>MKKLLPILIGLSLTGFSAMSQAENLLQVYQQARISNPDLRKSAADRDAAFEKINEARSPLLPQLGLGADYTYTSGFRDYKDQNSNVTSGSLQLTQVLFDMSKWRALTLQEKAAGIQDVTYQTDQQTLILNTATAYFKVLAAIDTLSYTEAQKQAIYRQLDQTTQRFNVGLVAITDVQNARSQYDAVLANEVTARNDLDNAVEELRQVTGNYYPELASLNVDGFKTSKPQAVNALLKEAENRNLSLLQARLNQDLAREQIRQAQDGHLPTLDLNASSGVSNNRYSGSKSISQDADIGQNKIGLSFSLPLYQGGMVNSQVKQAQYNFVGASEQLESAHRSVVQTVRSSFNNVNASISSINAYKQAVVSAQSSLDAMEAGYSVGTRTIVDVLDATTTLYNAKQQLSNARYNYLINELNIKSALGTLNEQDLIALNNTLGKPISTSADSVAPENPQQDATADGYGNTTAAMKPASARTTTHSSGSNPFRQLEHHHHHH[3x];> MADNQPVPLTPAPPGMVSLGVNENGEEEMTVIGGDGSGTGFSGNEAPIIPGSGSLQADLGKKSLTRLQAESSAAIHATAKWTTENLAKTQAAQAERAKAAMLSQQAAKAKQAKLTQHLKDVVDRALQNNKTRPTVIDLAHQNNQQMAAMAEFIGRQKAIEEARKKAEREAKRAEEAYQAALRAQEEEQRKQAEIERKLQEARKQEAAAKAKAEADRIAAEKAEAEARAKAEAERRKAEEARKALFAKAGIKDTPGCLEHHHHHH

Here, we use biochemical, biophysical and structural analyses to show how a bacteriocin exploits TolC, a major outer-membrane antibiotic efflux channel in Gram-negative bacteria, to transport itself across the outer membrane of target cells. Klebicin C (KlebC), a rRNase toxin produced by Klebsiella pneumoniae, binds TolC of a related species (K. quasipneumoniae) with high affinity through an N-terminal, elongated helical hairpin domain common amongst bacteriocins. TolC is one of the most prevalent drug efflux channels in bacteria and is frequently associated with multidrug resistance. Our results indicate that TolC, in addition to its known role in antibiotic export, can function as a protein import channel for bacteriocins.

Application of symmetry during processing then allowed for symmetry expansion of the dataset and subtraction of particles to give a single monomer, after which 3D sorting of particles revealed several classes where KlebC density was weakly apparent. A single class was further processed (see “Methods” and Supplementary Fig. 5) to produce the final 3.1 Å map of the TolC trimer with both helix 1 and 2 of KlebC resolved. In the final model, density corresponding to helix 1 and the N-terminal end of helix 2 of a single KlebC molecule span 109 Å of the TolC lumen; the N-terminal end of helix 1 is located near the periplasmic iris of TolC while helix 2 resides near the top within the outer-membrane β-barrel. The conformation of KlebC observed within the complex demonstrates unequivocally that the KlebC hairpin unfurls, forming a distorted kinked structure in which helix 1 is positioned against the α-helical region of TolC, and residues 137–151 form helix 2 within the transmembrane β-barrel of TolC. By contrast, in the complex with KqTolC this region forms the N-terminal end of helix 2. In contrast, helix 2 of KlebC packs against the β-barrel region of chain C with His140 and Gln141, from within interhelical linker, now forming hydrogen bonds to Ser68 and Asp47 of TolC, respectively. The N-terminus of KlebC helix 1 is oriented such that it is proximal to both chain A and C of the TolC trimer towards the iris, whilst the C-terminus of helix 1 can solely interact with chain A where the helices of TolC meet the β-barrel strands at the inner leaflet of the OM. The modelled structure of the complex shows charge complementarity plays an important role in stabilising the complex since several localised regions of positive and negative charge are matched. The unfurling of the KlebC1-254 helical hairpin required to bind TolC results in the loss of 1994 Å2 buried accessible surface area between the two helices. This is compensated for in the complex with TolC by the burial of 2384 Å2, predominantly through interactions with subunits A and C of TolC (1170 Å2 and 1120 Å2, respectively).N-myristoyltransferase (Nmt), which belongs to the GCN5 acetyltransferase superfamily, catalyzes the myriastate group from myristoyl-coenzyme A (myristoyl-CoA) to the N terminus or internal glycine residue of a protein by forming a covalent bond. This catalytic modification, reaction known as N-myristoylation, occurs in organism cotranslational or posttranslational processing. AflNmt is necessary for colony growth, spore germination, and sclerotia formation in A. flavus. The blots of AflNmt-GFP (green fluorescent protein) were found in the hyphal cytoplasm but did not overlap with those of the fluorescent nuclear dye (DAPI [4′,6-diamidino-2-phenylindole]) under luminescence microscope observation, suggesting that AlfNmt exercises its biological functions as a cytoplasmic protein.

With reference to the homologous protein in A. fumigatus, the truncated recombinant Nmt protein (Δ1-89 rAflNmt) was expressed as N-terminal Trx-6×His-fusion proteins in an E. coli strain. rAflNmt expression had a relatively low background level and a highly soluble yield in the E. coli expression system. Single peaks of elution fraction were detected from the chromatography profile, indicating that Δ1-89 rAflNmt is consistent with its theoretical molecular weight and exists solely as a monomer in elution buffer. By observing changes in the fluorescent substrate CPM [7-diethylamino-3-(4-maleimido-phenyl)-4-methylcoumarin], Δ1-89 rAflNmt was shown to possess N-myristoyltransferase catalytic activity. The rAflNmt crystal was diffracted to a high resolution of 1.78 Å and was in the P41 space group. The asymmetric unit contained only one rAflNmt molecule, and the structural model was refined to Rwork 0.23 and Rfree 0.26 with Ramachandran (favored 93.6%, allowed 5.1%, and outlier 1.28%). The approximate dimensions of spherical rAflNmt molecule are about 50 × 60 × 55 Å, and this protein is folded into a typical compact α/β topological shape similar to the GCN5-related N-acetyltransferase superfamily structure. In the N-terminal or C-terminal subunit, the core of the protein region is formed by several β-sheets and surrounded with a few α-helices. In comparison with other Nmt proteins, the myristoyl-CoA binding site and adjacent inhibitor binding pocket were found on the surface of the rAflNmt molecule. The AlphaFold2-calculated structure agreed very well overall with the experimental X-ray AflNmt structure. Major differences between these two structures occurred in the N-terminal region of the enzyme, including the following motifs: Ab loop, αD helix, βc, and βd.

> GPQTQPVPRFDETSNASGGPIKIIDPEKVSKEPDQLIEGFEWTTLDLTNETELQELWDLLTYHYVEDDNAMFRFRYSQSFLHWALMSPGWRKEWHVGVRATKSKKLVASICGVPTEIRVRDQKLKVTEINFLCIHKKLRSKRLTPVLIKEITRRCYLNGIYQAIYTAGVVLPTPVSSCRYYHRPLDWLKLYEVGFSPLPHGSTKARQITKNHLPSTTSTPGLRPMEIKDIDAVHDLLERYLKRFDMNQAFTKEEIEHWLVHKDGAGKEQVVWSYVVEDPETHKITDFFSFYNLPSTVIQHPKHKEVRAAYLYYYATETAFTEDLKALKERLLLLMNDALIQAKKAHFDVFNALTLHDNPLFLEQLKFGAGDGQLHFYLYNYRTAPIPGGVNEKNLPDEKKMGGVGVVML>[2x]AYTTFSQTKNDQLKEPMFFGQPVNVARYDQQKYDIFEKLIEKQLSFFWRPEEVDVSRDRIDYQALPEHEKHIFISNLKYQTLLDSIQGRSPNVALLPLISIPELETWVETWAFSETI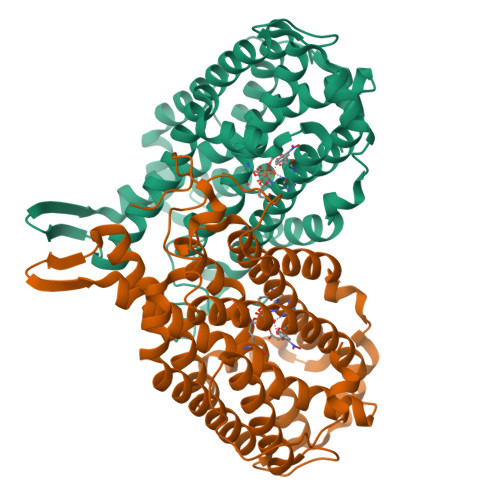HSRSYTHIIRNIVNDPSVVFDDIVTNEQIQKRAEGISSYYDELIEMTSYWHLLGEGTHTVNGKTVTVSLRELKKKLYLCLMSVNALEAIRFYVSFACSFAFAERELMEGNAKIIRLIARDEALHLTGTQHMLNLLRSGADDPEMAEIAEECKQECYDLFVQAAQQEKDWADYLFRDGSMIGLNKDILCQYVEYITNIRMQAVGLDLPFQTRSNPIPWINTWLVSDNVQVAPQEVEVSSYLVGQIDSEVDTDDLSNFQL> GGSYNDFGNYNNQSSNFGPMKGGNFG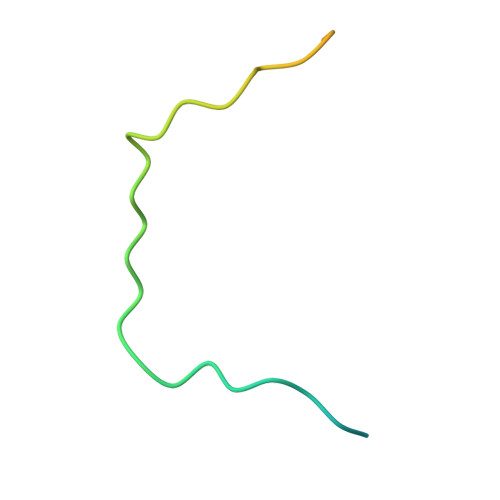GRSSGPYGGGGQYFAKPRNQGGY> GDRVADVIESSIGDSVSRALTQALPAPTGQNTQVSSHRLDTGEVPALQAAEIGASSNTSDESMIETRCVLNSHSTAETTLDSFFSRAGLVGEIDLPLEGTTNPNGYANWDIDITGYAQMRRKVELFTYMRFDAEFTFVACTPTGQVVPQLLQYMFVPPGAPKPESRESLAWQTATNPSVFVKLTDPPAQVSVPFMSPASAYQWFYDGYPTFGEHKQEKDLEYGACPNNMMGTFSVRNVGSSKSKYPLVVRIYMRMKHVRAWIPRPMRNQNYLFKANPNYAGNSIKPTGTSRTAITTLG;> SPSAEACGYSDRVAQLTIGNSTITTQEAANIIVGYGEWPSYCSDDDATAVDKPTRPDVSVNRFYTLDTKLWEKSSKGWYWKFPDVLTETGVFGQNAQFHYLYRSGFCIHVQCNASKFHQGALLVAILPEYVIGTVAGGTGTEDSHPPYKQTQPGADGFELQHPYVLDAGIPISQLTVCPHQWINLRTNNCATIIVPYMNTLPFDSALNHCNFGLLVVPISPLDFDQGATPVIPITITLAPMCSEFAGLRQAVTQ;> GFPTEPKPGTNQFLTTDDGVSAPILPNFHPTPCIHIPGEVRNLLELCQVETILEVNNVPTNATSLMERLRFPVSAQAGKGELCAVFRADPGRDGPWQSTMLGQLCGYYTQWSGSLEVTFMFTGSFMATGKMLIAYTPPGGPLPKDRATAMLGTHVIWDFGLQSSVTLVIPWISNTHYRAHARDGVFDYYTTGLVSIWYQTNYVVPIGAPNTAYIIALAAAQKNFTMKLCKDTSHILQTASIQ;> MGSQVSTQRSGS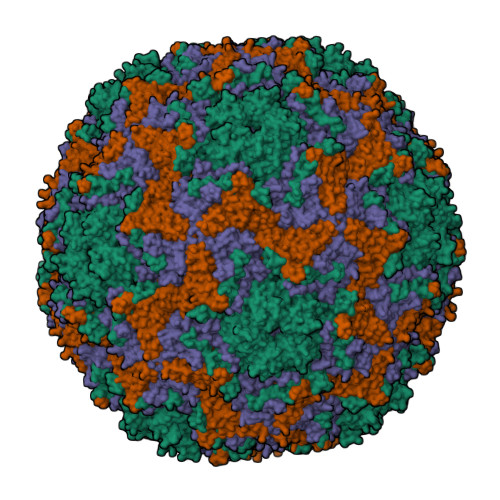HENSNSATEGSTINYTTINYYKDSYAATAGKQSLKQDPDKFANPVKDIFTEMAAPLK> SQIGLFSKICRVTIKTLHYYNKIGLLVPAYINPDNGYRFYTSDQLMKFHQIASLRQLGFTITEIVTLTQDENSCHIIERRRLEIQKQIRDMADMLSRINHYLQHKKKERIMLYQAALKEIPECIVYSKRFIVPDFSSYIKLIPPIGQEVMKANPGLTLTTPAYCFTL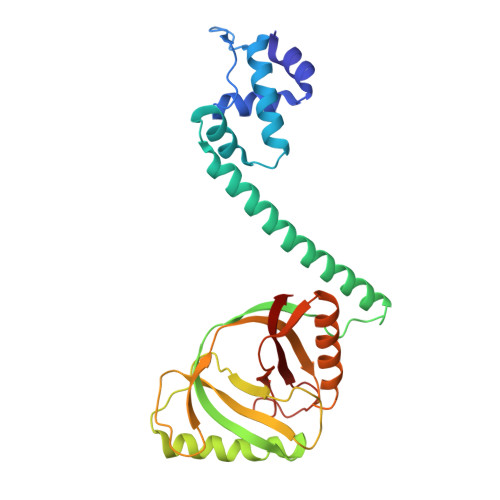YHDKEYKEKNMDVEFCEAVNDFGKNEGNIIFQVIPAITAVTVIHKGPYDSLRNAYIYLMQWVEDNGYLLTNSPRESYIDGIWNKQDSAEWMTEIQFPVEKV> APVRSLNCTLRDSQQKSLVMSGPYELKALHLQGQDMEQQVVFSMSFVQGEESNDKIPVALGLKEKNLYLSCVLKDDKPTLQLESVDPKNYPKKKMEKRF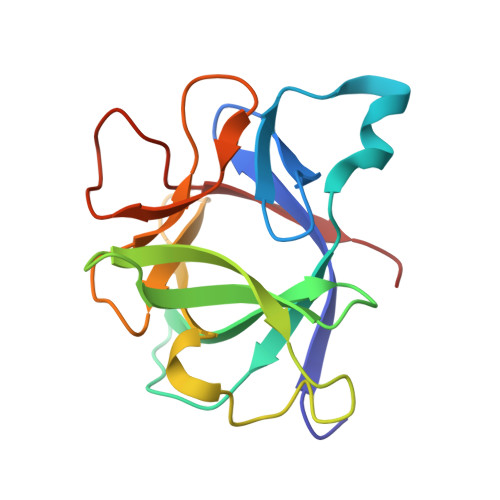VFNKIEINNKLEFESAQFPNWYISTSQAENMPVFLGGTKGGQDITDYTMQFVSS> MDLAKLGLKEVMPTKINLEGLVGDHAFSMEGVGEGNILEGTQEVKISVTKGAPLPFAF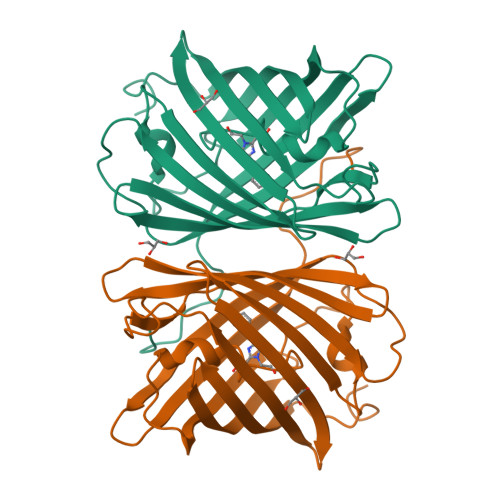DIVSVAFTYGNRAYTGYPEEISDYFLQSFPEGFTYERNIRYQDGGTAIVKSDISLEDGKFIVNVDFKAKDLRRMGPVMQQDIVGMQPSYESMYTNVTSVIGECIIAFKLQTGKHFTYHMRTVYKSKKPVETMPLYHFIQHRLVKTNVDTASGYVVQHETAIAAHSTIKKIEGSLP>[2x]SNAMLSPNVDTALNMLTDVYTDFLGISNYDATCNSLFIGHVAKDPNWLVEVRSRTEILRAVMNEFMQQKPKIFAQIITSFINYQTTFDACAQNSKAITSTKQWIECLQLLQKTLKQNITLTNEAQQVFTKSYNQAKNAEELLASSIQDGWNELASEEQAMVRIATEIGSLSQSIASLGANVTAAQLRAGKAYIQSMVTISYGVVMTTSVPFLS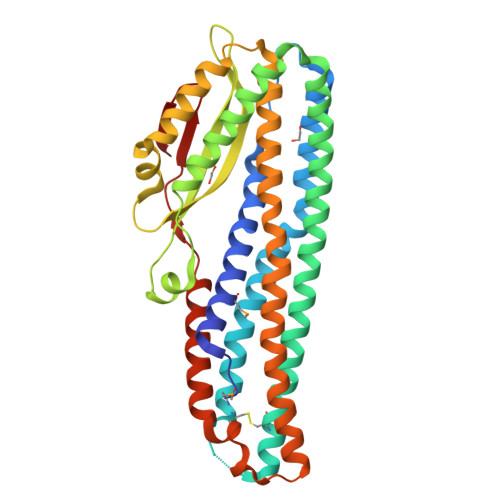FAGALFTVGYSAYSTISSAKEVQQDLDKLTQLQTLASEEAQAAAITKAIIQTLSNMSEEFLKIDDSLPALSLLWQDELDKVNELINALQSGSDPALLTDLQTIKIASASWKTISEFVQLISLPPNVGKPVLVNTLNNTIQEQ>[2x]MENTENSVDSKSIKNLE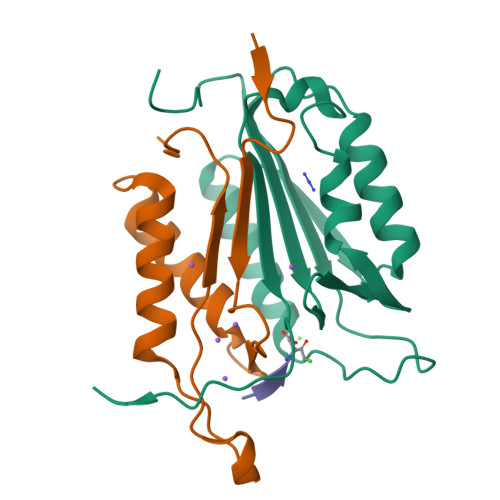PKIIHGSESMDSGISLDNSYKMDYPEMGLCIIINNKNFHKSTGMTSRSGTDVDAANLRETFRNLKYEVRNKNDLTREEIVELMRDVSKEDHSKRSSFVCVLLSHGEEGIIFGTNGPVDLKKITNFFRGDRCRSLDGKPKLFIIQACRGTELDCGIETD;>[2x]SGVDDDMACHKIPVEADFLYAYSTAPGYYSWRNSKDGSWFIQSLCAMLKQYADKLEFMHILTRVNRKVATEFESFSFDATFHAKKQIPCIVSMLTKELYFYH>MHHHHHHGSDDDDKRPEAKSAQPADGWKGERPRSEEDNELN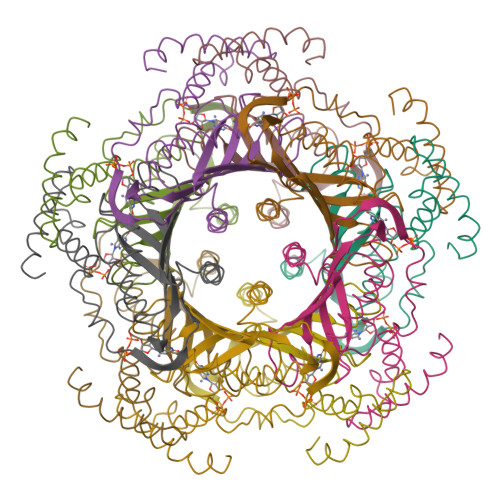LPNLAAAYSSILSSLGENPQRQGLLKTPWRAASAMQFFTKGYQETISDVLNDAIFDEDHDEMVIVKDIDMFSMCEHHLVPFVGKVHIGYLPNKQVLGLSKLARIVEIYSRRLQVQERLTKQIAVAITEALRPAGVGVVVEATHMCMVMRGVQKMNSKTVTSTMLGVFREDPKTREEFLTLIRS[20x]>MSELEKAVVALIDVFHQYSGREGDKHKLKKSELKELINNELSHFLEEIKEQEVVDKVMETLDSDGDGECDFQE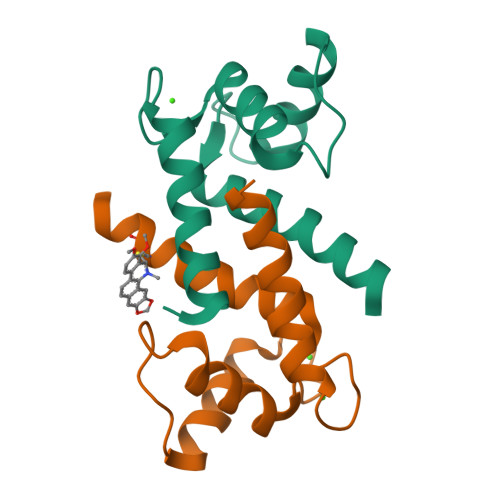FMAFVAMITTACHEFFEHE[2x]>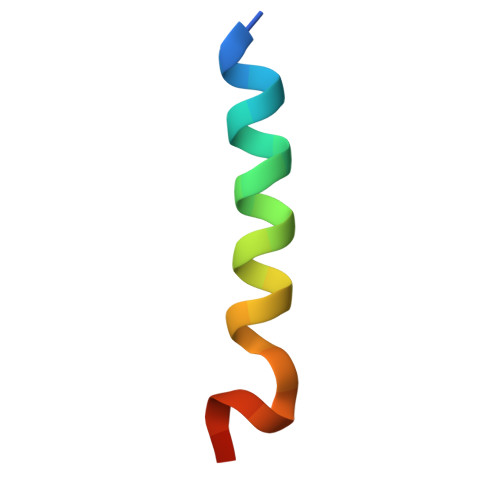 GAMGSVEHTLADVLYHVETEVENLYFQ>MEYTQLGRIGLKVSRLVLGTMNFGPTTDEAESHAIMDAALDAGINFFDTANVYGWGENKGRTEEILGSWFAQGGDRRDKVVLATKVYGNMGLDGPAWPNHDKLSALNIRRSVDASLKRLGTDHIDLYQFHHVDRDTPWDEIWQAMDVLVRQGKILYVGSSNFAGWNIAQANETAARHGRLGLVSEQCLYNLCERRAEMEVVPAAREYGLGVIAWSPLHGGLLGGAIRKEQEGGNRRAASGRAADALKDPQQREQIQRYEDLLDKHGLEPGEVALAWLLTRPGVTGPIVGPRTADQLASAVRAAELTLTDEVLTALDEIFPGPGPSPEAFAW[16x]

Aldo-keto reductases (AKRs) are a superfamily of oxidoreductases capable of reducing carbonyl to primary and secondary alcohols, found in all phyla. In this work, we identify the enzyme AKRtyl, which is responsible for tylosin reduction. Phylogenetic analysis indicates that AKRtyl is the founding member of subfamily D within family 12 in the AKR superfamily. Specifically, by combining steady-state and transient kinetics, X-ray crystallography and molecular dynamics simulation, we demonstrate that AKRtyl exhibits a positive synergy mediated by an unusual Monod-Wyman-Changeux (MWC) paradigm of allosteric regulation at low concentrations of the cofactor NADPH, but an inhibitory effect at high concentrations is observed.

To obtain the apo structure of AKRtyl, we remove the carried cofactors by denaturation and refolding. We successfully obtained two apo structures of AKRtyl without any cofactor. The first apo structure is similar to our previous second purified-state structure, with two octamers in an asymmetric unit and one active (R4) and one dormant (T4) tetramer per octamer (R4T4). Unlike the classical MWC model where different conformational equilibria occur in the actual oligomeric state, AKRtyl is actually octameric, but we observe symmetric T and R conformational equilibria within the tetramer. We therefore propose that the basic unit of MWC-type allosteric ensemble is a tetramer rather than an octamer for: (1) The tetramer exhibits ligand-independent T and R conformations, suggesting that the equilibrium between the T and R conformations occurs within the tetramer.(3S,4S,5R)-3-(4-amino-3-{[(2R)-3-ethoxy-1,1,1-trifluoropropan-2-yl]oxy}-5-fluorobenzyl)-5-[(3-tert-butylbenzyl)amino]tetrahydro-2H-thiopyran-4-ol 1,1-dioxide | C28 H38 F4 N2 O5 S 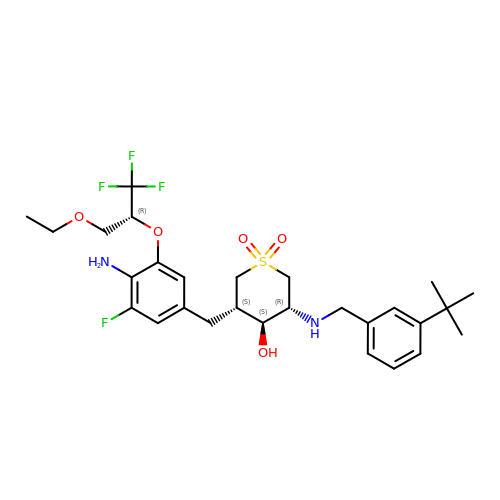| UJZFSYZNJMWXJO-NJONLQHESA-N> MALISQSIKNLKGGISQQPDILRYPDQGSRQVNGWSSETEGLQKRPPLVFLNTLGDNGALGQAPYIHLINRDEHEQYYAVFTGSGIRVFDLSGNEKQVRYPNGSNYIKTANPRNDLRMVTVADYTFIVNRNVVAQKNTKSVNLPNYNPNQDGLINVRGGQYGRELIVHINGKDVAKYKIPDGSQPEHVNNTDAQWLAEELAKQMRTNLSDWTVNVGQGFIHVTAPSGQQIDSFTTKDGYADQLINPVTHYAQSFSKLPPNAPNGYMVKIVGDASKSADQYYVRYDAERKVWTETLGWNTEDQVLWETMPHALVRAAD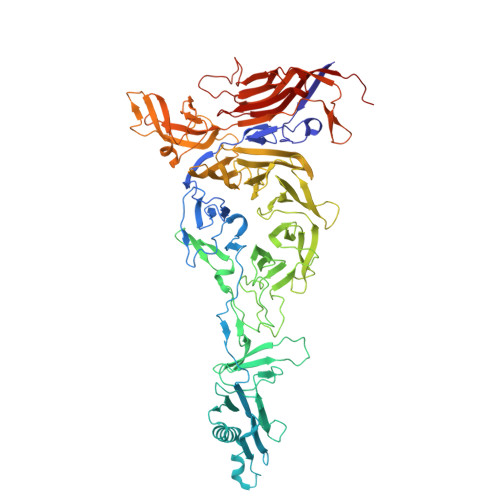GNFDFKWLEWSPKSCGDVDTNPWPSFVGSSINDVFFFRNRLGFLSGENIILSRTAKYFNFYPASIANLSDDDPIDVAVSTNRIAILKYAVPFSEELLIWSDEAQFVLTASGTLTSKSVELNLTTQFDVQDRARPFGIGRNVYFASPRSSFTSIHRYYAVQDVSSVKNAEDITSHVPNYIPNGVFSICGSGTENFCSVLSHGDPSKIFMYKFLYLNEELRQQSWSHWDFGENVQVLACQSISSDMYVILRNEFNTFLARISFTKNAIDLQGEPYRAFMDMKIRYTIPSGTYNDDTFTTSIHIPTIYGANFGRGKITVLEPDGKITVFEQPTAGWNSDPWLRLSGNLEGRMVYIGFNINFVYEFSKFLIKQTADDGSTSTEDIGRLQLRRAWVNYENSGTFDIYVENQSSNWKYTMAGARLGSNTLRAGRLNLGTGQYRFPVVGNAKFNTVYILSDETTPLNIIGCGWEGNYLRRSSGI> MKRMLAEFEKIQAILMAFPHEFSDWAYCIKEARESFLNIIQTIAKHAKVLVCVHTNDTIGYEMLKNLPGVEIAKVDTNDTWARDFGAISIENHGVL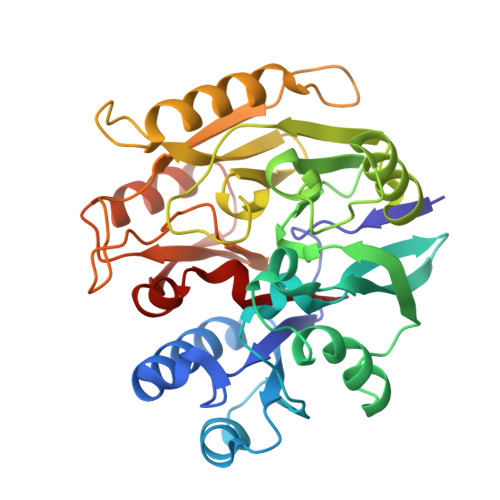ECLDFGFNGWGLKYPSNLDNQVNFKLKSLGFLKHPLKTMPYVLEGGSIESDGAGSILTNTQCLLEKNRNPHLNQNGIETMLKKELGAKQVLWYSYGYLKGDDTDSHTDTLARFLDKDTIVYSACEDKNDEHYTALKKMQEELKTFKKLDKTPYKLIPLEIPKAIFDENQQRLPATYVNFLLCNDALIVPTYNDPKDALILETLKQHTPLEVIGVDCNTLIKQHGSLHCVTMQLY>[2x]DYTVHDTDGKPVLNNAGQYYILPA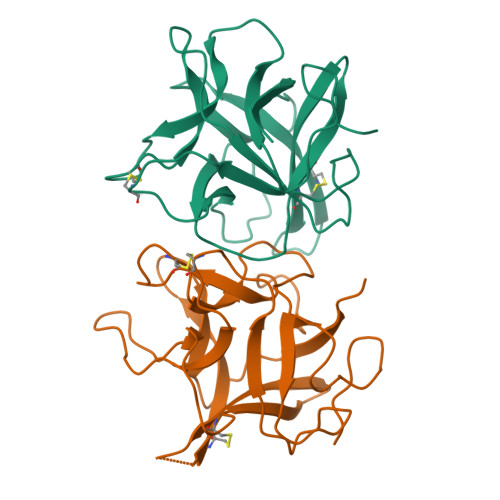KQGKGGGLGLSNDDDGNCPLTVSQTPIDLPIGLPVRFSSRARISHITTALSLNIEFTIAPACAPKPARWRIFNEQSSEKGYTPVKISDDFSSAAPFQIKKFEEDYKLVYCSKSESGERKCVDLGIKIDDEKNRRLVLKEGDPFKVKFKKVDEESSEEWSIV> VDDVTGEKVREAFEQFLEDFSVQSTDTGEVEKVYRAQIEFMKIYDLNTIYIDYQHLSMRENGALAMAISEQYYRFLPFLQKGLRRVVRKYAPXXXXXXXXXXXXXXERVFQISFFNLPTVHRIRDIRSEKIGSLLSISGTVTRTSEVRPELYKASFTCDMCRAIVDNVEQSFKYTEPTFCPNPSCENRAFWTLNVTRSRFLDWQKVRIQENANEIPTGSMPRTLDVILRGDSVERAKPGDRCKFTGVEIVVPDVTQLGLPGVKPSSTLDTRGISKTTEGLNSGVTGLRSLGVRDLTYKISFLACHVISIGXXXXXXXXXXXXXXXXXXXXXXXXXXSDEINELKEMVKDEHIYDKLVRSIAPAVFGHEAVKKGILLQMLGGVHKSTVEGIKLRGDINICVVGDPSTSKSQFLKYVVGFAPRSVYTSGKASSAAGLTAAVVRDEEGGDYTIEAGALMLADNGICCIDEF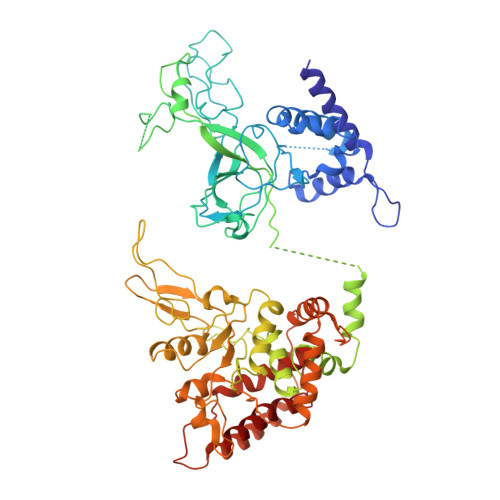DKMDISDQVAIHEAMEQQTISIAKAGIHATLNARTSILAAANPVGGRYNRKLSLRGNLNMTAPIMSRFDLFFVILDDCNEKIDTELASHIVDLHMKRDEAIEPPFSAEQLRRYIKYARTFKPILTKEARSYLVEKYKELRKDDAQGFSRSSYRITVRQLESMIRLSEAIARANCVDEITPSFIAEAYDLLRQSIIRVDV> MGSDKIHHHHHHENLYFQGMSIEERLEALEKEIQKMKDIE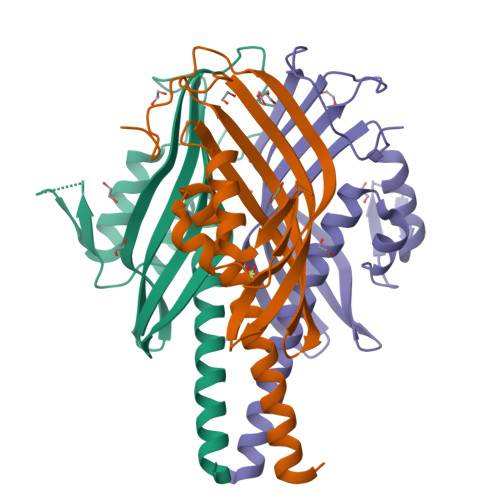EIKKLKGQYFRCLDGKFWDELETTLSPNIVTSYSNGKLVFHGPKEVTDYFKKAMPREEISMHMGHTPEITIDSETTATGRWYLEDKLIFTEESKYAGSGVNGGAFYTDKYEKVDGKWYILETGYLRVYEEHFMRDPKIKITMNMHKTK> GYKYKQKPKYQVRWKIIESYEGNSYTFIDPTQLPYNEKWEFPRNNLQFGKTLGAGAFGKVVEATAFGLGKEDAVLKVAVKMLKSTAHADEKEALMSELKIMSHLGQHENIVNLLGACTHGGPVLVITEYCC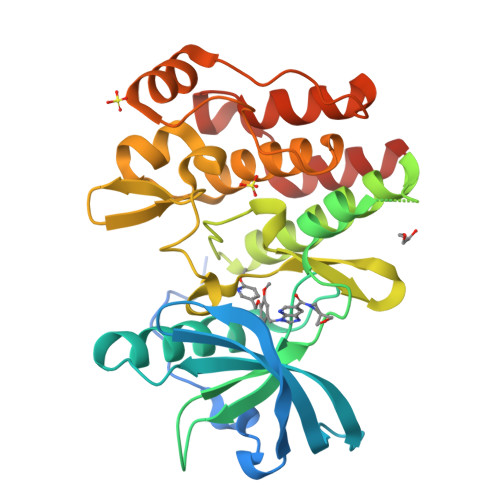YGDLLNFLRRKRPPGLEYSYNPSHNPEEQLSSRDLLHFSSQVAQGMAFLASKNCIHRDVAARNVLLTNGHVAKIGDFGLARDIMNDSNYIVKGNARLPVKWMAPESIFDCVYTVQSDVWSYGILLWEIFSLGLNPYPGILVNSKFYKLVKDGYQMAQPAFAPKNIYSIMQACWALEPTHRPTFQQICSFLQEQAQEDRRERD HP activity is regulated by its first and rate-limiting enzyme glutamine fructose-6-phosphate amidotransferase (GFAT, EC 2.6.1.16). GFAT is a modular enzyme composed of a glutaminase domain responsible for hydrolysis of l-Gln into l-glutamate (l-Glu) and an isomerase/transferase domain that catalyzes the isomerization of Frc6P to glucose-6-phosphate (Glc6P) as well as the transfer of ammonia to Glc6P to build glucosamine-6-phosphate (GlcN6P). The relative orientation of the two domains with their respective active sites is relevant for catalysis and affected by substrate binding. GFAT-1 activity is modulated by UDP-GlcNAc feedback inhibition and via phosphorylation by protein kinase A (PKA).

The well-conserved C-tail (C-terminal residues 670–681) is the major mobile element between the isomerase and glutaminase domain of GFAT. To independently test whether thermal shift assays can indeed indicate domain interactions, we generated the C-tail lock mutant L405R of human GFAT-1 and characterized it structurally, as well as in thermal shift assays and in kinetic measurements. Miszkiel and Wojciechowski showed in molecular dynamic simulations that the C-tail lock mutation, which introduces a salt-bridge similar as observed in E. coli, limits the C-tail’s flexibility. We solved the crystal structure (resolution 2.38 Å) and confirmed that the L405R substitution indeed formed a salt-bridge with the C-terminal Glu681 and additionally interacted with Asp428. The kinetics (l-Gln and Frc6P) and the UDP-GlcNAc inhibition remained unaffected by the C-tail lock mutation. Importantly, the L405R mutant clearly showed a single melting point at 56.9 ± 0.1 °C in thermal shift assays, indicating a changed stability of both domains, which can only be explained by the altered interactions between them. Therefore, thermal shift assays are a valid tool to analyze domain interactions of GFAT-1.

>MCGIFAYLNYHVPRTRREILETLIKGLQRLEYRGYDSAGVGFDGGNDKDWEANACKIQLIKKKGKVKALDEEVHKQQDMDLDIEFDVHLGIAHTRWATHGEPSPVNSHPQRSDKNNEFIVIHNGIITNYKDLKKFLESKGYDFESETDTETIAKLVKYMYDNRESQDTSFTTLVERVIQQLEGAFALVFKSVHFPGQAVGTRRGSPLLIGVRSEHKLSTDHIPILYRTGKDKKGSCNLSRVDSTTCLFPVEEKAVEYYFASDASAVIEHTNRVIFLEDDDVAAVVDGRLSIHRIKRTAGHHHHHHDHPGRAVQTLQMELQQIMKGNFSSFMQKEIFEQPESVVNTMRGRVNFDDYTVNLGGLKDHIKEIQRCRRLILIACGTSYHAGVATRQVLEELTELPVMVELASDFRDRNTPVFRDDVCFFLSQSGETADTLMGLRYCKERGALTVGITNTVGSSISRETDCGVHINAGPEIGVASTKAYTSQFVSLVMFALMMCDDRISMQERRKEIMLGLKRLPDLIKEVLSMDDEIQKLATELYHQKSVLIMGRGYHYATCLEGALKIKEITYMHSEGILAGELKHGPLALVDKLMPVIMIIMRDHTYAKCQNALQQVVARQGRPVVICDKEDTETIKNTKRTIKVPHSVDCLQGILSVIPLQLLAFHLAVLRGYDVDFPRNLAKSVTVE[2x]>[2x]GSSHHHHHHSSGLVPRGSPQPPADEQPEPRTRRRAYLWCKEFLPGAWRGLREDEFHISVIRGGLSNMLFQCSLPDTTATLGDEPRKVLLRLYGAILQMRSCNKEGSEQAQKENEFQGAEAMVLESVMFAILAERSLGPKLYGIFPQGRLEQFIPSRRLDTEELSLPDISAEIAEKMATFHGMKMPFNKEPKWLFGTMEKY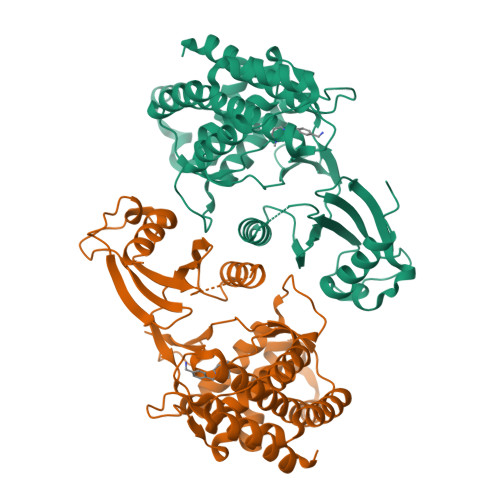LKEVLRIKFTEESRIKKLHKLLSYNLPLELENLRSLLESTPSPVVFCHNDCQEGNILLLEGRENSEKQKLMLIDFEYSSYNYRGFDIGNHFCEWMYDYSYEKYPFFRANIRKYPTKKQQLHFISSYLPAFQNDFENLSTEEKSIIKEEMLLEVNRFALASHFLWGLWSIVQAKISSIEFGYMDYAQARFDAYFHQKRKLGV> MRVNNGLTPQELEAYGISDVHDIVYNPSYDLLYQEELDPSLTGYERGVLTNLGAVAVDTGIFTGRSPKDKYIVRDDTTRDTFWWADKGKGKNDNKPLSPETWQHLKGLVTRQLSGKRLFVVDAFCGANPDTRLSVRFITEVAWQAHFVKNMFIRPSDEELAGFKPDFIVMNGAKCTNPQWKEQGLNSENFVAFNLTERMQLIGGTWYGGEMKSGMFSMMNYLLPLKGIASMHCSANVGEKGDVAVFFGLSGTGKTTLSTDPKRRLIGDDEHGWDDDGVFNFEGGCYAKTIKLSKEAEPEIYNAIRRDALLENVTVREDGTIDFDDGSKTENTRVSYPIYHIDNIVKPVSKAGHATKVIFLTADAFGVLPPVSRLTADQTQYHFLSGFTAKLAGTERGITEPTPTFSACFGAAFLSLHPTQYAEVLVKRMQAAGAQAYLVNTGWNGTGKRISIKDTRAIIDAILNGSLDNAETFTLPMFNLAIPTELPGVD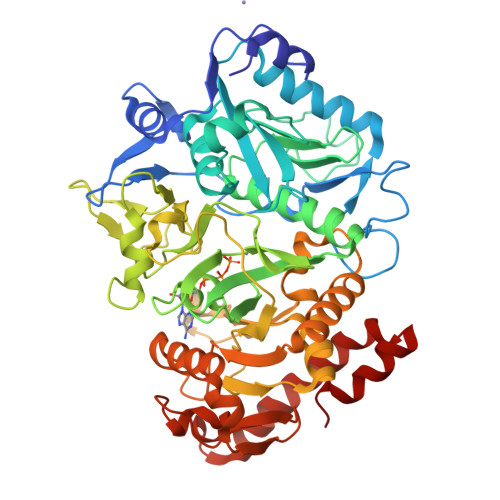TKILDPRNTYASPEQWQEKAETLAKLFIDNFDKYTDTPAGAALVAAGPKL> L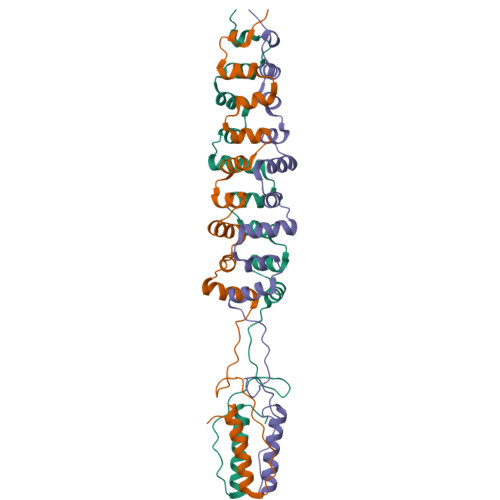VISRSKEISIEVEDIKDAGDTGKRLLKINTPSGARNIIIENEDAKALINGETTNTNKKNLQDLLFSDGNVKAFLQATTTDENKTALQQLLVSNADVLGLLSGNPTSDNKINLRTMIGAGVPYSLPAATTTTLGGVKKGAAVTASTATDVATAVKDLNSLITVLKNAGIISLEHHHHHH>[4x]MSQQPGVLPENMKRYMGRDAQRMNILAGRIIAETVRSTLGPKGMDKMLVDDLGD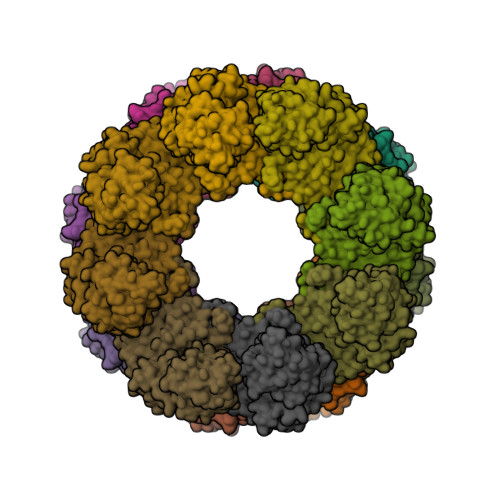VVVTNDGVTILREMSVEHPAAKMLIEVAKTQEKEVGDGTTTAVVVAGELLRKAEELLDQNVHPTIVVKGYQAAAQKAQELLKTIACEVGAQDKEILTKIAMTSITGKGAEKAKEKLAEIIVEAVSAVVDDEGKVDKDLIKIEKKSGASIDDTELIKGVLVDKERVSAQMPKKVTDAKIALLNCAIEETASEMLKDMVAEIKASGANVLFCQKGIDDLAQHYLAKEGIVAARRVKKSDMEKLAKATGANVITNIKDLSAQDLGDAGLVEERKISGDSMIFVEECKHPKAVTMLIRGTTEHVIEEVARAVDDAVGVVGCTIEDGRIVSGGGSTEVELSMKLREYAEGISGREQLAVRAFADALEVIPRTLAENAGLDAIEILVKVRAAHASNGNKCAGLNVFTGAVEDMCENGVVEPLRVKTQAIQSAAESTEMLLRIDDVIAAEKLRGAPDMGDMGGMPGMGGMPGMM>MIGEITTFFGMRVFTDEGRYVGRVEDVILDQNTKSIRGLAISDYNKALIDSHAKGVIIPYRVVKAVGDIIIIKDLFKRKSRVLDYESRELIE[2x];>[4x]MYVPARSLARKSVVLTDGTVVGTLYNITVDFKTGTIVNLLVKPENEIPDFKKEEGLYIIPFECVRSLKDFIVVDRR;>[2x]MIGEITTFFGMRVFTDEGRYVGRVEDVILDQNTK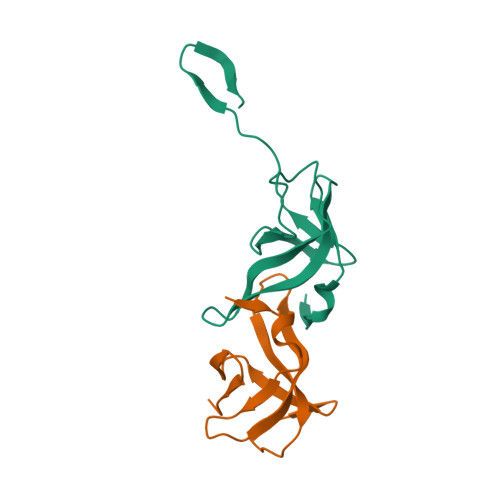SIRGLAISDYNKALIDSHAKGVIIPYRVVKAVGDIIIIKDLF The first step of the incorporation pathway involves the activation of sialic acid to a cytidine monophosphate diester form catalyzed by CMP-sialic acid synthetase (EC 2.7.7.43), a ubiquitous enzyme that is found in both prokaryotes and eukaryotes. In the presence of Mg2+, CMP-sialic acid synthetase (CMAS) catalyzes a sequential ordered reaction that involves a nucleophilic attack on the α-phosphate of CTP by the anomeric O atom of β-Neu5Ac and the production of CMP-sialic acid and pyrophosphate (PPi). The activated sialic acid is then incorporated into LOS or LPS by sialyltransferases. In this report, we present crystal structures of the apo form of the VcCMAS enzyme and of that complexed with cytidine diphos­phate (CDP) and Mg2+.

The orthorhombic crystals (space group P212121) of the CDP-bound enzyme contain four molecules in the asymmetric unit arranged as dimer of dimers (AB and CD). The final refined CDP-bound VcCMAS model contains protein residues 3–228 in subunits A and D, 0–233 in subunit B and 1–227 in subunit C plus three CDP molecules, one Mg2+ ion, one Ca2+ ion and one tetraethylene glycol (PG4), one triethylene glycol (PGE) and two ethylene glycol (EDO) molecules. The P-loop residues 13–20 are disordered in subunit D, which lacks CDP in the active site. The nucleotide-binding residues in subunit C and the bound CDP molecule (CDP 1) have well ordered electron density with low temperature factors and thus were used in structural analyses. Hydrogen-bond interactions between the conserved Arg71 guanidium Nη1 and Nη2 atoms and the N3 and O5 atoms of the cytosine base impart selectivity of the enzyme towards CTP. Several conserved residues in the P loop such as Arg12, Gly14, Ser15, Lys16 and Lys21 interact with the α- and β-phosphoryl groups of the nucleotide. c electron density indicative of a metal ion close to the α-phosphate of CDP and the putative Mg2+-binding residues Asp213 and Asp215 (analogous to Asp209 and Asp211 in NmCMAS) in protomer C. Along with the Mg2+ ion at this site, several water molecules interacting with the phosphoryl group of the nucleotide and the metal ion were also identified. Since the Mg2+ ion interacts with both the protein and the α-phosphoryl group of CDP and is situated adjacent to the catalytic 2′-OH group of the modeled Neu5Ac, we designate this Mg2+ ion as the catalytic ion that is responsible for activating the hydroxyl group of Neu5Ac. Upon CDP binding, the VcCMAS structure shows conformational changes in the dimerization domain, which lead to partial closure of the active site and place the catalytic Arg169 near the Neu5Ac binding pocket. As a consequence, the CDP-bound VcCMAS monomers have a larger dimer interface (1699 Å2) compared with the apo structure (1429 Å2).

>MHHHHHHITSLYKKAGFMSNEYVALITARGGSKGLLRKNVLPLHGIPLIGWTIKAAQGCSYISKVFVSTDDYEIAKISEGLGALVINRPEELATDTASSIDVILHAISWLEQKEVQKYEGMILLQPTSPLRTSHHIKEAIELYEKTAAKFVISVFEPTHTPIKSYLENDDGTISGLYSNEAPYQRRQDLPRAYQPNGAIYAFSIDEFKLNNHFPRNKVFPYVMSEVESADIDTLEDLRKVEEQLKIKEINK[4x]>[5x]PVDVSVSIFINKIYGVNTLEQTYKVDGYIVAQWTGKPRKTPGDKPLIVENTQIERWINNGLWVPALEFINVVGSPDTGNKRLMLFPDGRVIYNARFLGSFSNDMDFRLFPFDRQQFVLELEPFSYNNQQLRFSDIQVYTENIDNEEIDEWWIR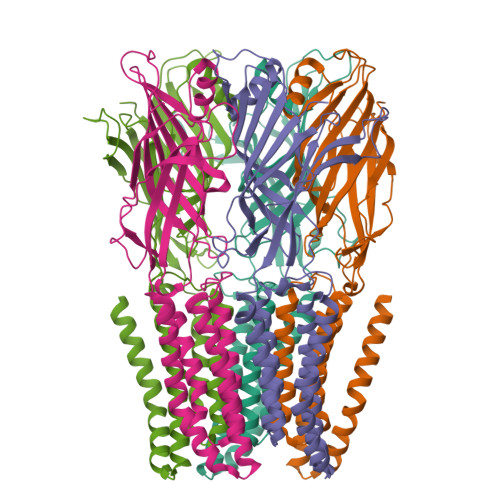GKASTHISDIRYDHLSSVQPNQNEFSRITVRIDAVRNYFSYIPNIILPMLFILFISWTAFWSTSYEANVTLVVSTLIAHIAFNILVETNLPKTPYMTYTGAIIFMIYLFYFVAVIEVTVQHYLKVESQPARAASITRASRIAFPVVFLLANIILAFLFF> PSLRKQRFMQFSSLEHEGEYYMTPRDFLFSVMFEQMERKTSVKKLTKKDIEDTLSGIQTAGCGSTFFRDLGDKGLISYTEYLFLLTILTKPHSGFHVAFKMLDTDGNEMIEKREFFKLQKIISKQDDLMTVKTNETGYQEAIVKEPEINTTLQMRFFGKRGQRKLHYKEFRRFMENLQTEIQEMEFLQFSKGLSFM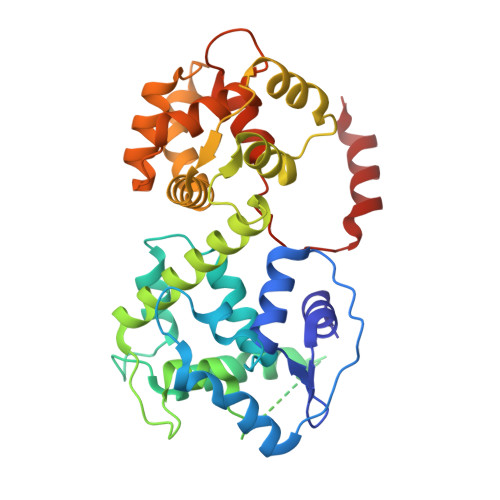RKEDFAEWLLFFTNTENKDIYWKNVREKLSAGESISLDEFKSFCHFTTHLEDFAIAMQMFSLAHRPVRLAEFKRAVKVATGQELSNNILDTVFKIFDLDGDECLSHEEFLGVLKNRMHRGLWVPQHQSIQEYWKCVKKES>GPGSDTERPVVNVPSEITVYRGESFEYFATVTDNSNAFDLAKTVVRWLYSNQPGRGTEWLQYSVTQVGNQLKVRIFGNVPIDTTIGDYTRYVVATDAAGNVNATQTEMGNAAVDKTSVNGQFKLII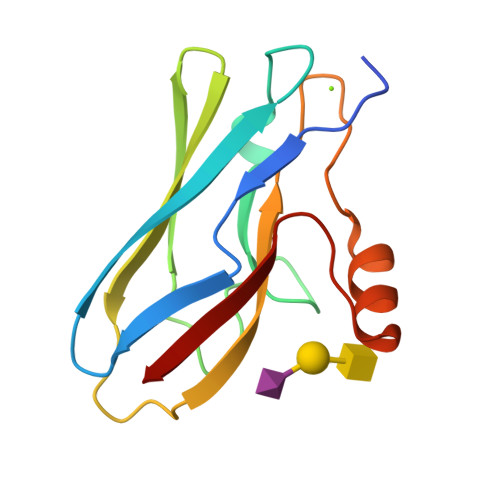R[2x]> GHMRLELPVIPLRNTVILPHTTTPVDVGRAKSKRAVEEAMGADRLIFLVAQRDPEVDDPAPDDLYTWGVQAVVKQAMRLPDGTLQVMVEARARAQVTDYIPGPYLRARGEVFSEIFPIDEAVVRVLVEELKEAFEKYVANHKSLRLDRYQLEAVKGTSDPAMLADTIAYHATWTVAEKQEILELTDLEARLKKVLGLLSRDLERFELDKRVAQRVKEQMDTNQREYYLREQMKAIQKELGGEDGLSDLEALRKKIEEVGMPEAVKTKALKELDRLERMQQGSPEATVARTYLD

The Lon AAA+ protease (LonA) is a ubiquitous ATP-dependent proteolytic machine, which selectively degrades damaged proteins or native proteins carrying exposed motifs (degrons). LonA belongs to the AAA+ (ATPases associated with various cellular activities) superfamily and contains an N-terminal domain (NTD), a middle ATPase domain with conserved Walker motifs for ATP hydrolysis, and a C-terminal protease domain (CTD) with a serine-lysine catalytic dyad in the active site. Substrate recognition of LonA is thought to be mediated by its NTD. Collectively, our results showed that the NTD of LonA selectively interacts with protein substrates via critical hydrophobic residues of its N-lobe, demonstrating that the NTD enables LonA to perform protein quality control by selectively interacting with proteins in damaged or unfolded states.

Based on the result, we also crystallized and solved the structure of the longer N-terminal fragment NN291. The structure of NN291, refined to 1.7 Å resolution, is very similar to that of NN206 except for a longer C-terminal helix by four more residues, that is, residues 207–210. Despite the lack of spontaneous proteolytic fragmentation in the crystals, no electron density was seen past residue A210. (D) The refined 2Fo-Fc electron density map around the C-terminal residue A210 of NN291, contoured at 1.0 σ. Nonetheless, NN243 exhibited extra intense and poorly dispersed cross-peaks around 7.5–8.5 ppm along the proton dimension that is indicative of a highly disordered peptide segment, which most likely corresponds to the C-terminal extension of NN243. Together, our crystallographic and NMR analyses suggest that the NTD of MtaLonA forms a bilobal globular structure (residues 1–206) followed by a C-terminal flexible extension (residues 211–243). Our crystallographic results of NN206 and NN291 are consistent with previous findings that the ~40 residue region between the NTD and ATPase–Protease domains is structurally flexible with multiple accessible protease sites. We further applied multidimensional heteronuclear NMR experiments to assign the observed cross-peaks in 1H–15N TROSY-HSQC spectrum of NN206 (BMRB code: 50697) and the NMR-derived secondary structure of NN206, based on the Chemical Shift Index, was highly similar to its solved X-ray structures. Together, these results suggested that in a MtaLonA complex, each of the six NTDs may connect to the hexameric core by a flexible ~40-residue linker.> MRVLLIHADYFEYEVKDKALKNPEPISEDMKRGRMEEVLVAFISVEKVDEKNPEEVSLKAIEEISKVAEQVKAENVFVSPWAHLSSELAKPSVAMDILNRVYQGLKERGFNVGKAPFGYYIAVKISCKGHPL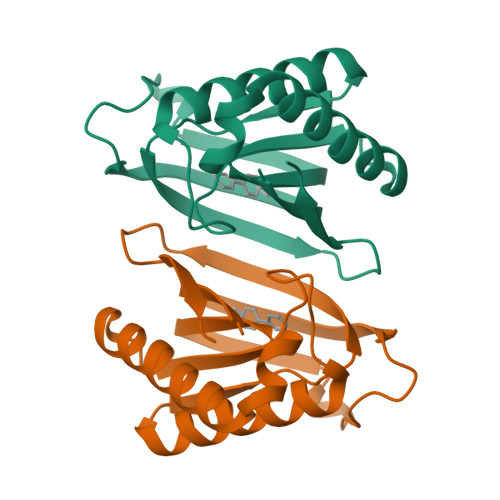AELSRTIVPEELEHHHHHH>MSLTIKNSLGQSHDYIKMFVKEGDTVVDATCGNGNDTAFLASLVGENGRVFGFDIQDKAIANTTKKLTDLNLIDRVTLIKDGHQNMDKYIDCPVKAVMFNLGYLPSGDHSISTRPETTIQALSKAMELLVTGGIITVVIYYGGDTGFEEKEKVLEFLKGVD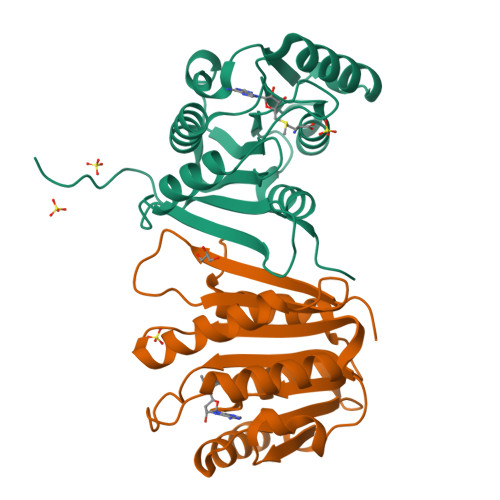QKKFIVQRTDFINQANCPPILVCIEKISEGHHHHHH[10x]> DAGTVDFYGQLRTELKFLEDKDPTIGSGSSRAGVDANYTVNDSLALQGKVEFALKDSGDMYVRNHILGVKTNFGKFSFGKQWTTSDDVYGADYSYFFGGTGLRYGTLSDALHDSQVKYVYEADSFWVKAGYGFPEDNAKQELAELYVGATFGDLAVHAGGGQNRDKAFKVGSNTVGTTTTDIKADVTNSY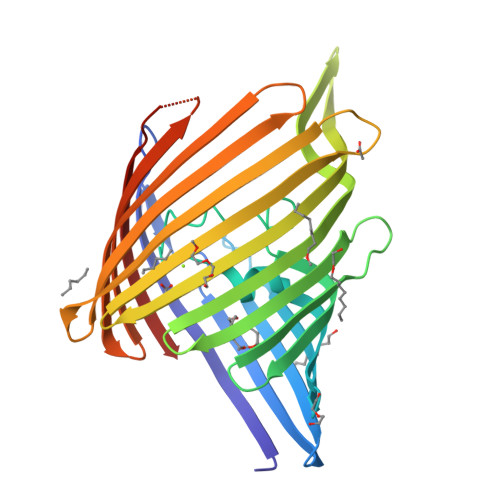FEVTGEYTIGDALIGVTYYNAELDVENNPLVIDEDAISVAGTYKVADKTKLYAGYEYVMQEANTGADEDGTLVYLGVEYKFASWARVYAEYGYGDGTTLGYTNKGSDAEVKATKGDSANNFGIGARYYW> PQQQSAFKQLYTELFNNEGDFSKVSSNLKKPLKCYVKESYPHFLVTDGYFFVAPYFTKEAVNEFHAKFPNVNIVDLTDKVIVINNWSLELRRVNSAEVFTSYANLEARLIVHSFKPNLQERLNPTRYPVNLFRDDEFKTTIQHFRHTALQAAI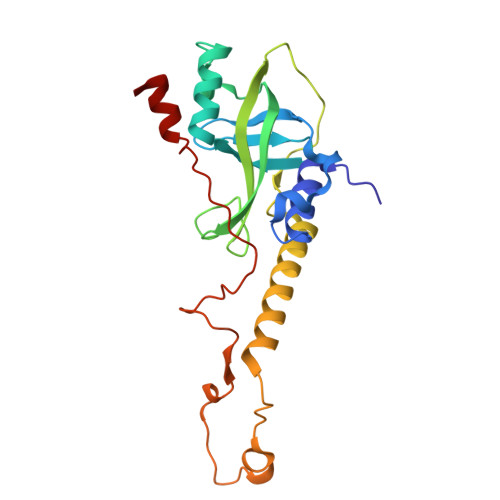NKTVKGDNLVDISKVADAAGKKGKVDAGIVKASASKGDEFSDFSFKEGNTATLKIADIFVQEKG>[2x]VDSVYRTRSLGVAAEGIPDQYADGEAARVWQLYIGDTRSRTAEYKAWLLGLLRQHGCHRVLDVACGTGVDSIMLVEEGFSVTSVDASDKMLKYALKERWNRRKEPAFDKWV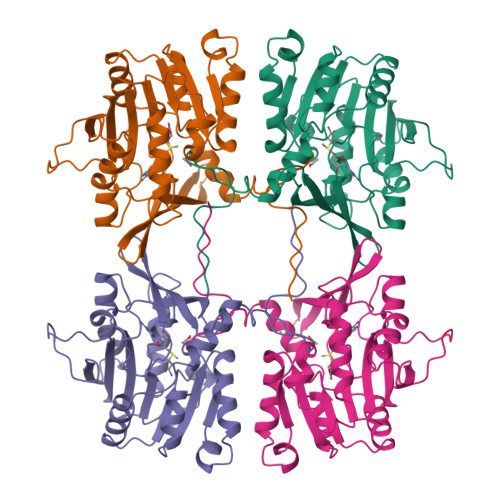IEEANWLTLDKDVPAGDGFDAVICLGNSFAHLPDSKGDQSEHRLALKNIASMVRPGGLLVIDHRNYDYILSTGCAPPGKNIYYKSDLTKDITTSVLTVNNKAHMVTLDYTVQVPGAGRDGAPGFSKFRLSYYPHCLASFTELVQEAFGGRCQHSVLGDFKPYRPGQAYVPCYFIHVLKKTG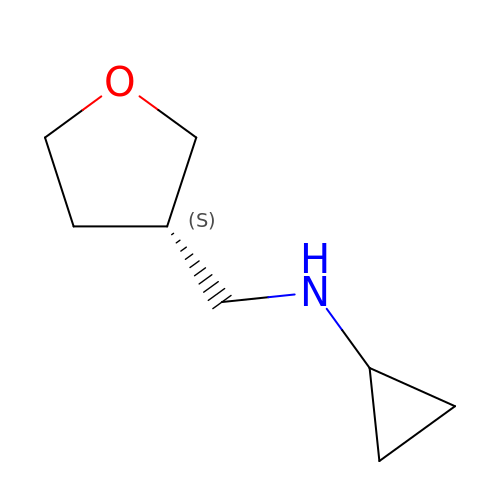~{N}-[[(3~{S})-oxolan-3-yl]methyl]cyclopropanamine | C8 H15 N O | XTBAPHZUOIOBDQ-ZETCQYMHSA-N CNG channels open when bound with cGMP and conduct Na+ and Ca2+ ions into photoreceptor cells. The gating ring transmits cGMP binding/unbinding-triggered conformational changes in the CNBD to the TMD, where a cavity gate formed by two hydrophobic residues in S6 opens and closes. Cryo-EM structures of the Caenorhabditis elegans TAX-4 CNG channel carrying the analogous mutation, R421W, show that most apo channels are open. R421W disrupts this interaction, destabilizes the closed state, and stabilizes the open state.

Surprisingly, consensus 3D refinement of apo TAX-4_R421W cryo-EM single particles revealed substantial heterogeneity and suggested the existence of channels in both closed and open states. Further processing with an S6-gating ring-CNBD mask and focused 3D classification showed that indeed apo TAX-4_R421W existed not only in the closed state but also in an open state; the two structures were determined at 3.2 and 3.1 Å resolution, respectively, with C4 symmetry. The closed-state structures of apo TAX-4_R421W and apo WT TAX-4 are identical, with an r.m.s.d. of 0.50 Å when all visible amino acids are compared. In the closed state, R421 forms a salt bridge with E298 in S4 of a neighboring subunit; it also forms a hydrogen bond with Q425 in the A’ α helix and a cation-π interaction with W456 in the B’ α helix of the gating ring of the same subunit. The R421-E298 salt bridge is the only interaction between R421 and the transmembrane segments. The R421W mutation alters these interactions. In particular, the closed state is greatly destabilized due to the disruption of the R421-E298 intersubunit salt bridge and the resulting repulsion between the π system of W421 and the negative charge of E298. The intrasubunit R421-Q425 hydrogen bond and R421-W456 cation-π interaction observed in the closed state are also disrupted by the R421W mutation, albeit W421 still makes van der Waals contacts with Q425 and W456.

>[4x]GGGGSMSTAEPAPDPTNPSTSGLAPTTNGIGSPPPTASAATKFSILTKFLRRKNQVHTTTAQQNEFMQKYMPNGNSNAVQPAATGGQPASSDGGSAIEVPPPKESYAVRIRKYLANYTQDPSTDNFYYWTCVVTVAYIYNLLFVIARQVFNDLIGPSSQSLCRFYNGTLNSTTQVECTYNMLTNMKEMPTYSQYPDLGWSKYWHFRMLWVFFDLLMDCVYLIDTFLNYRMGYMDQGLVVREAEKVTKAYWQSKQYRIDGISLIPLDYILGWPIPYINWRGLPILRLNRLIRYKRVRNCLERTETRSSMPNAFRVVVVVWYIVIIIHWNACLYFWISEWIGLGTDAWVYGHLNKQSLPDDITDTLLRRYVYSFYWSTLILTTIGEVPSPVRNIEYAFVTLDLMCGVLIFATIVGNVGSMISNMSAAWTEFQNKMDGIKQYMELRKVSKQLEIRVIKWFDYLWTNKQSLSDQQVLKVLPDKLQAEIAMQVHFETLRKVRIFQDCEAGLLAELVLKLQLQVFSPGDFICKKGDIGREMYIVKRGRLQVVDDDGKKVFVTLQEGSVFGELSILNIAGSKNGNRRTANVRSVGYTDLFVLSKTDLWNALREYPDARKLLLAKGREILKKDNLLDENAPEEQKTVEEIAEHLNNAVKVLQTRMARLIVEHSSTEGKLMKRIEMLEKHLSRYKALARRQKTMHGVSIDGGDISTDGVDERVRPPRLRQTKTIDLPTGTESESLLK(1R,3R,7E,17beta)-17-[(2R)-5-hydroxypentan-2-yl]-2-methylidene-9,10-secoestra-5,7-diene-1,3-diol 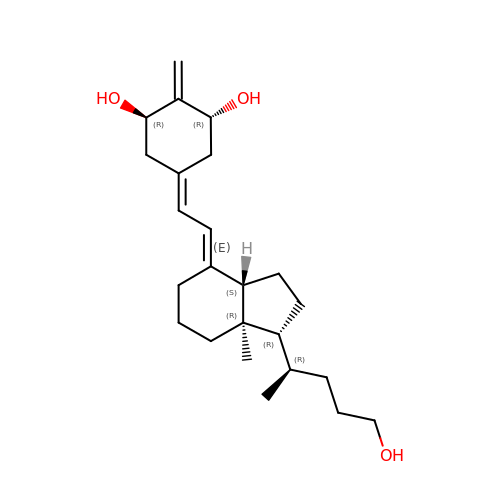| C24 H38 O3 | JPGZPBYJMAWTHF-HCMYXCKPSA-N> HMDIRPRLRIGQINLGGAEDATRELPSIARDLGLDIVLVQEQYSMVGFLAQCGAHPKAGVY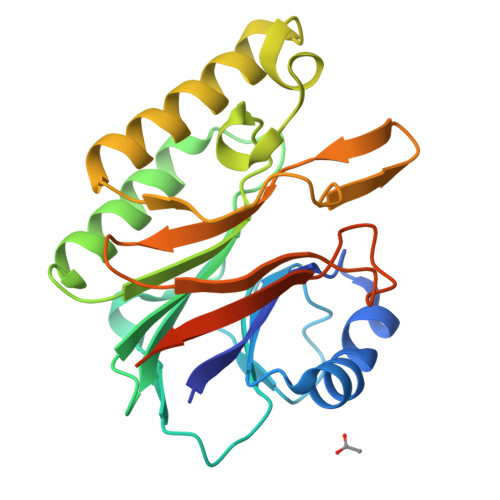IRNRVLPCAVLHHLSSTHITVVHIGGWDLYMVSAYFQYSDPIDPYLHRLGNILDRLRGARVVICADTNAHSPLWHSLPRHYVGRGQEVADRRAKMEDFIGARRLVVHNADGHLPTFSTANGESYVDVTLSTRGVRVSEWRVTNESSSDHRLIVFGVGGGTTGERDEDEEARSDLRPGEP>[2x]VQEPLRVPPSAPARLVVLASGTGSLLRSLLDAAVGDYPARVVAVGVDRECRAAEIAAEASVPVFTVRLADHPSRDAWDVAITAATAAHEPDLVVSAGFMRILGPQF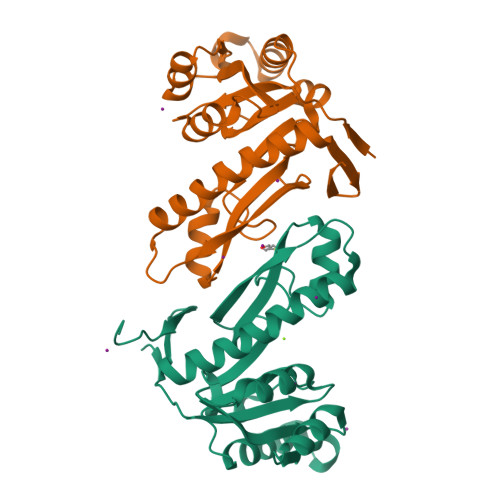LSRFYGRTLNTHPALLPAFPGTHGVADALAYGVKVTGATVHLVDAGTDTGPILAQQPVPVLDGDDEETLHERIKVTERRLLVAAVAALATHGVTVVGRTATMGRKVTIG>[3x]MFEARLVQGSILKKVLEALKDLINEACWDISSSGVNLQSMDSSHVSLVQLTLRSEGFDTYRCDRNLAMGVNLTSMSKILKCAGNEDIITLRAEDNADTLALVFEAPNQEKVSDYEMKLMDLDVEQLGIPEQEYSCVV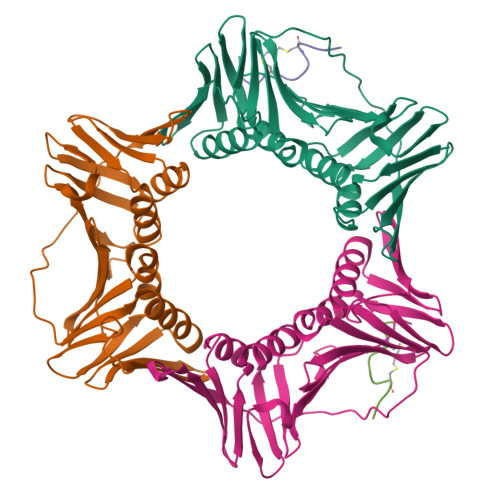KMPSGEFARICRDLSHIGDAVVISCAKDGVKFSASGELGNGNIKLSQTSNVDKEEEAVTIEMNEPVQLTFALRYLNFFTKATPLSSTVTLSMSADVPLVVEYKIADMGHLKYYLAPKIEDEE;>XRQCSMTCFYHSKX[2x]>MAHHHHHHRTIKVAINGFGRIGRLVFRSLLSKANVEVVAINDLTQPEVLAHLLKYDSAHGELKRKITVKQNILQIDRKKVYVFSEKDPQNLPWDEHDIDVV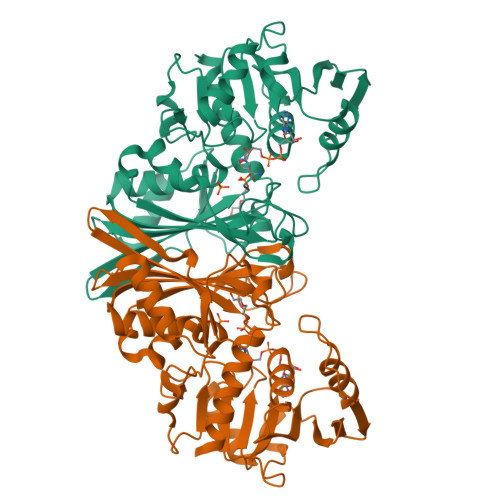IESTGRFVSEEGASLHLKAGAKRVIISAPAKEKTIRTVVYNVNHKTISSDDKIISAASCTTNCLAPLVHVLEKNFGIVYGTMLTVHAYTADQRLQDAPHNDLRRARAAAVNIVPTTTGAAKAIGLVVPEANGKLNGMSLRVPVLTGSIVELSVVLEKSPSVEQVNQAMKRFASASFKYCEDPIVSSDVVSSEYGSIFDSKLTNIVEVDGMKLYKVYAWYDNESSYVHQLVRVVSYCAKL[4x]(5BETA)-PREGNANE-3,20-DIONE | 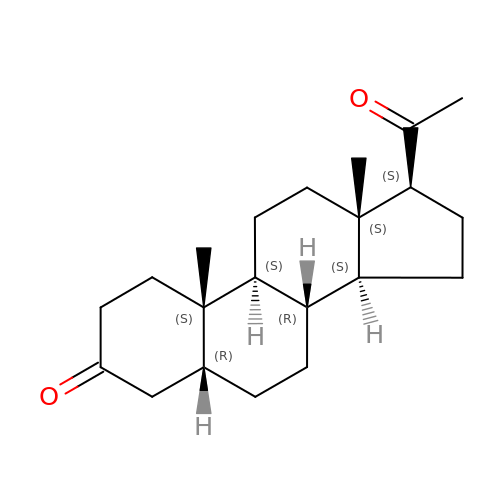C21 H32 O2 | XMRPGKVKISIQBV-XWOJZHJZSA-N> GSMVEATAQETDRPRFSFSIAAREGKARTGTIEMKRGVIRTPAFMPVGTAATVKALKPETVRATGADIILGNTYHLMLRPGAERIAK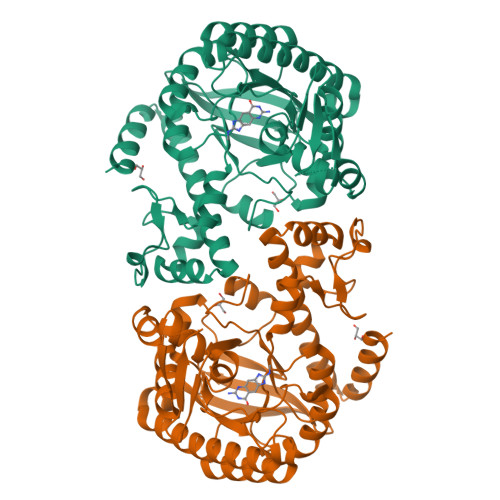LGGLHSFMGWDRPILTDSGGYQVMSLSSLTKQSEEGVTFKSHLDGSRHMLSPERSIEIQHLLGSDIVMAFNECTPYPATPSRAASSMERSMRWAKRSRDAFDSRKEQAENAALFGIQQGSVFENLRQQSADALAEIGFDGYAVGGLAVGEGQDEMFRVLDFSVPMLPDDKPHYLMGVGKPDDIVGAVERGIDMFDCVLPTRSGRNGQAFTWDGPINIRNARFSEDLKPLDSECHCAVCQKWSRAYIHHLIRAGEILGAMLMTEHNIAFYQQLMQKIRDSISEGRFSQFAQDFRARYFARNS>[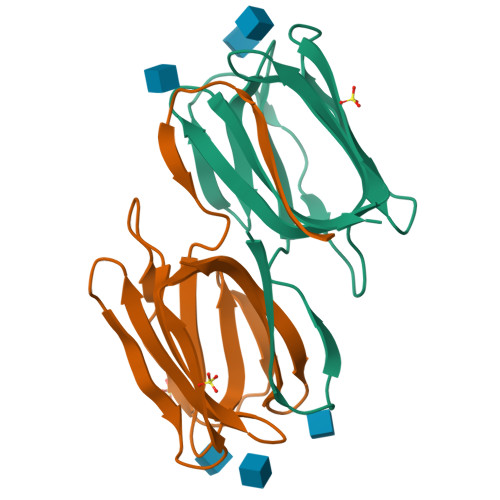2x]XSLTHRKFGGSGGSPFSGLSSIAVRSGSYLDAIIIDGVHHGGSGGNLSPTFTFGSGEYISNMTIRSGDYIDNISFETNMGRRFGPYGGSGGSANTLSNVKVIQINGSAGDYLDSLDIYYEQY The type III-E CRISPR-Cas system is a newly identified bifunctional complex with nuclease activity and protease activity that holds great potential for RNA editing applications. Here, we report cryo-electron microscopy (cryo-EM) structures of Desulfonema ishimotonii (Di) Cas7-11-crRNA, complexed with or without the full length or the N-terminus of TPR-CHAT. The Cas7 domains, arranged in a row, form a crescent-shaped filament, with the INS and CTE domain completing the structure. The Cas11 domain is positioned at the crescent’s midpoint, and interacts with Cas7.2 and Cas7.3.

The truncated TPR-CHAT containing only the NTD can independently interact with the complex at the same position. When the DiCas7-11-crRNA complex bound to DiTPR-CHAT or DiTPR-CHATNTD, the conformation of the DiCas7-11-crRNA complex was unchanged. The enhanced stability of Cas7.4 (V1317-R1336) is attributed to the formation of numerous interactions with DiTPR-CHATNTD. These interactions include a pair of salt bridges formed between Cas7.4 E1330 and TPR-CHATNTD R64, four pairs of hydrogen bonds formed between Cas7.4 L1333 and TPR-CHATNTD L50, Cas7.4 L1334, and TPR-CHATNTD R53, and Cas7.4 E1330 and TPR-CHATNTD R64 (two pairs), and dozens of pairs of nonbonded contacts. In contrast, the mutations of the NTD residues Q47A and G49A that formed hydrogen bonds with S1352 and H1337, respectively, outside of the segment of V1317-R1336 in Cas7.4 neither affected the formation of the complex nor the inhibitory activity of DiTPR-CHATNTD. We found that the affinity of the DiCas7-11-crRNA complex to the target RNA was reduced by the presence of full length (F) or NTD of DiTPR-CHAT but unaffected by the CTD. The regulatory characterization of DiTPR-CHATNTD by preventing target RNA binding to Cas protein is similar to anti-CRISPR proteins (Acrs). However, it is noteworthy that the activity of DiTPR-CHATNTD has only been demonstrated in vitro, and whether it can exert a similar inhibitory effect in vivo, particularly in mammalian cells, requires further study.

> MTTTMKISIEFLEPFRMTKWQESTRRNKNNKEFVRGQAFARWHRNKKDNTKGRPYITGTLLRSAVIRSAENLLTLSDGKISEKTCCPGKFDTEDKDRLLQLRQRSTLRWTDKNPCPDNAETYCPFCELLGRSGNDGKKAEKKDWRFRIHFGNLSLPGKPDFDGPKAIGSQRVLNRVDFKSGKAHDFFKAYEVDHTRFPRFEGEITIDNKVSAEARKLLCDSLKFTDRLCGALCVIRFDEYTPAADSGKQTENVQAEPNANLAEKTAEQIISILDDNKKTEYTRLLADAIRSLRRSSKLVAGLPKDHDGKDDHYLWDIGKKKKDENSVTIRQILTTSADTKELKNAGKWREFCEKLGEALYLKSKDMSGGLKITRRILGDAEFHGKPDRLEKSRSVSIGSVLKETVVCGELVAKTPFFFGAIDEDAKQTDLQVLLTPDNKYRLPRSAVRGILRRDLQTYFDSPCNAELGGRPCMCKTCRIMRGITVMDARSEYNAPPEIRHRTRINPFTGTVAEGALFNMEVAPEGIVFPFQLRYRGSEDGLPDALKTVLKWWAEGQAFMSGAASTGKGRFRMENAKYETLDLSDENQRNDYLKNWGWRDEKGLEELKKRLNSGLPEPGNYRDPKWHEINVSIEMASPFINGDPIRAAVDKRGTDVVTFVKYKAEGEEAKPVCAYKAESFRGVIRSAVARIHMEDGVPLTELTHSDCECLLCQIFGSEYEAGKIRFEDLVFESDPEPVTFDHVAIDRFTGGAADKKKFDDSPLPGSPARPLMLKGSFWIRRDVLEDEEYCKALGKALADVNNGLYPLGGKSAIGYGQVKSLGIKGDDKRISRLMNPAFDETDVAVPEKPKTDAEVRIEAEKVYYPHYFVEPHKKVEREEKPCGHQKFHEGRLTGKIRCKLITKTPLIVPDTSNDDFFRPADKEARKEKDEYHKSYAFFRLHKQIMIPGSELRGMVSSVYETVTNSCFRIFDETKRLSWRMDADHQNVLQDFLPGRVTADGKHIQKFSETARVPFYDKTQKHFDILDEQEIAGEKPVRMWVKRFIKRLSLVDPAKHPQKKQDNKWKRRKEGIATFIEQKNGSYYFNVVTNNGCTSFHLWHKPDNFDQEKLEGIQNGEKLDCWVRDSRYQKAFQEIPENDPDGWECKEGYLHVVGPSKVEFSDKKGDVINNFQGTLPSVPNDWKTIRTNDFKNRKRKNEPVFCCEDDKGNYYTMAKYCETFFFDLKENEEYEIPEKARIKYKELLRVYNNNPQAVPESVFQSRVARENVEKLKSGDLVYFKHNEKYVEDIVPVRISRTVDDRMIGKRMSADLRPCHGDWVEDGDLSALNAYPEKRLLLRHPKGLCPACRLFGTGSYKGRVRFGFASLENDPEWLIPGKNPGDPFHGGPVMLSLLERPRPTWSIPGSDNKFKVPGRKFYVHHHAWKTIKDGNHPTTGKAIEQSPNNRTVEALAGGNSFSFEIAFENLKEWELGLLIHSLQLEKGLAHKLGMAKSMGFGSVEIDVESVRLRKDWKQWRNGNSEIPNWLGKGFAKLKEWFRDELDFIENLKKLLWFPEGDQAPRVCYPMLRKKDDPNGNSGYEELKDGEFKKEDRQKKLTTPWTPWA;> NPIRDIQDRLKTAKFDNKDDMMNLASSLYKYEKQLMDSSEATLCQQGLSNRPNSFSQLSQFRD> CCGCCUAACACUGCCAAUGCCGGUCCCAAGCCCGGAUAAAAGUGG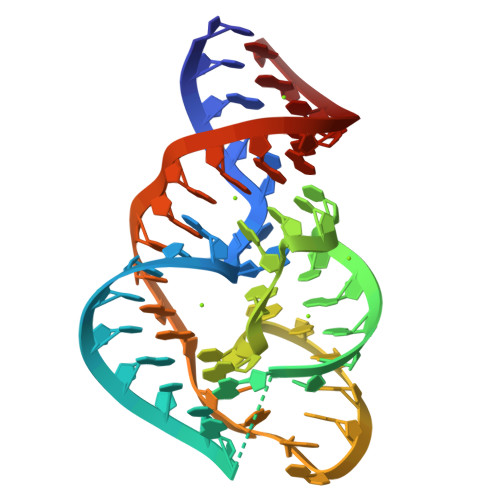AGGGGGCGG> MRCIGISNRDFVEGVSGGSWVDIVLEHGSCVTTMAKNKPTLDFELIKTEAKQPATLRKYCIEAKLTNTTTDSRCPTQGEPTLNEEQDKRFVCKHSMVDRGWGNGCGLFGKGGIVTCAMFTCKKNMEGKIVQPENLEYTVVITPHSGEEHAVGNDTGKHGKEVKITPQSSITEAELTGYGTVTMECSPRTGLDFNEMVLLQMKDKAWLVHRQWFLDLPLPWLPGADTQGSNWIQKETLVTFKNPHAKKQDVVVLGSQEGAMHTALTGATEIQMSSGNLLFTGHLKCRLRMDKLQLKGMSYSMCTGKFKVVKEIAETQHGTIVIRVQYEGDGSPCKIPFEIMDLEKRHVLGRLITVNPIVTEKDSPVNIEAEPPFGDSYIII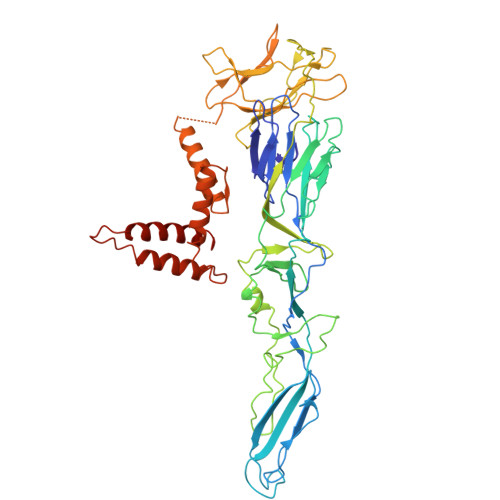GVEPGQLKLDWFKKGSSIGQMFETTMRGAKRMAILGDTAWDFGSLGGVFTSIGKALHQVFGAIYGAAFSGVSWTMKILIGVIITWIGMNSRSTSLSVSLVLVGIVTLYLGVMVQA> GPHMLEPAATVDHSQRICEVWACNLDEEMKKIRQVIRKYNYVAMDTEFPGVVARPIGEFRSNADYQYQLLRCNVDLLKIIQLGLTFMNEQGEYPPGTSTWQFNFKFNLTEDMYAQDSIELLTTSGIQFK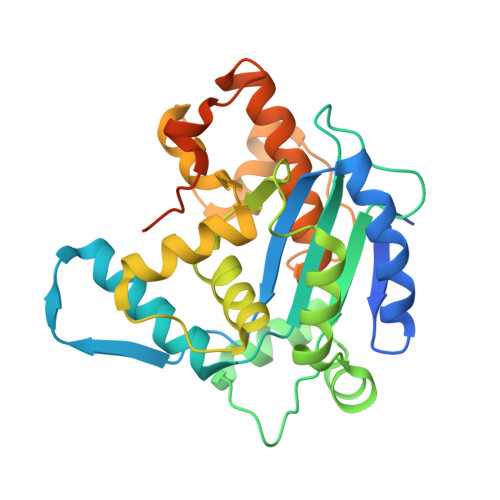KHEEEGIETQYFAELLMTSGVVLCEGVKWLSFHSGYDFGYLIKILTNSNLPEEELDFFEILRLFFPVIYDVKYLMKSCKNLKGGLQEVAEQLELERIGPQHQAGSDSLLTGMAFFKMREMFFEDHIDDAKYCGHLYGLGSGSSYVQNGTGNAYEEEANKQS> 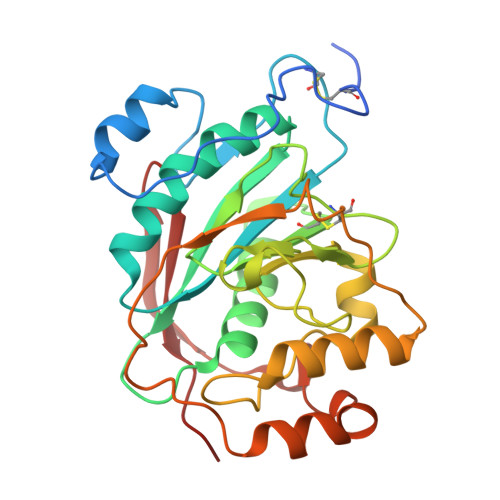ASMTGGQQMGRGSSLTACPEESPLLVGPMLIEFNIPVDLKLVEQQNPKVKLGGRYTPMDCISPHKVAIIIPFRNRQEHLKYWLYYLHPILQRQQLDYGIYVINQAGESMFNRAKLLNVGFKEALKDYDYNCFVFSDVDLIPMNDHNTYRCFSQPRHISVAMDKFGFSLPYVQYFGGVSALSKQQFLSINGFPNNYWGWGGEDDDIYNRLAFRGMSVSRPNAVIGKTRHIRHSRDKKNEPNPQRFDRIAHTKETMLSDGLNSLTYMVLEVQRYPLYTKITVDIGTPS>MRVLALSAVFLVASIIGMPAVAKEWQ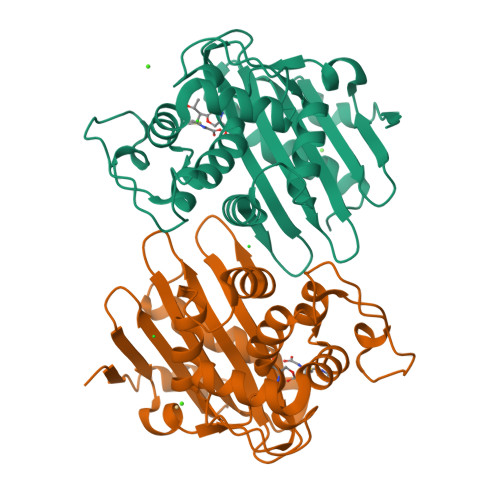ENKSWNAHFTEHKSQGVVVLWNENKQQGFTNNLKRANQAFLPASTFKIPNSLIALDLGVVKDEHQVFKWDGQTRDIATWNRDHNLITAMKYSVVPVYQEFARQIGEARMSKMLHAFDYGNEDISGNVDSFWLDGGIRISATEQISFLRKLYHNKLHVSERSQRIVKQAMLTEANGDYIIRAKTGYSTRIEPKIGWWVGWVELDDNVWFFAMNMDMPTSDGLGLRQAITKEVLKQEKIIP[2x]4-(2-AMINO-5-{4-[(DIMETHYLAMINO)METHYL]THIOPHEN-2-YL}PYRIDIN-3-YL)-2-{[(1R,2Z)-4,4,4-TRIFLUORO-1-METHYLBUT-2-EN-1-YL]OXY}BENZAMIDE 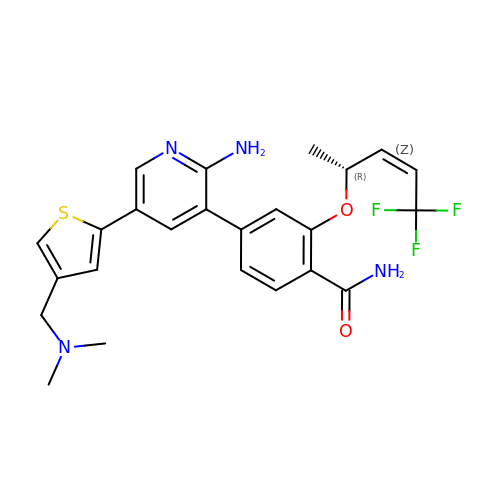| C24 H25 F3 N4 O2 S | LLEOOSLUHRQCHZ-LMVHVUTASA-N> MEKVFYVTTPIYYVNAEPHLGHAYTTVVADFLARWHRLDGYRTFFLTGTDEHGETVYRAAQAAGEDPKAFVDRVSGRFKRAWDLLGIAYDDFIRTTEERHKKVVQLVLKKVYEAGDIYYGEYEGLYCVSCERFYTEKELVEGLCPIHGRPVERRKEGNYFFRMEKYRPWLQEYIQENPDLIRPEGYRNEVLAMLAEPIGDLSISRPKSRVPWGIPLPWDENHVTYVWFDALLNYVSALDYPEGEAYRTFWPHAWHLIGKDILKPHAVFWPTMLKAAGIPMYRHLNVGGFLLGPDGRKMSKTLGNVVDPFALLEKYGRDALRYYLLREIPYGQDTPVSEEALRTRYEADLADDLGNLVQRTRAMLFRFAEGRIPEPVAGEELAEGTGLAGRLR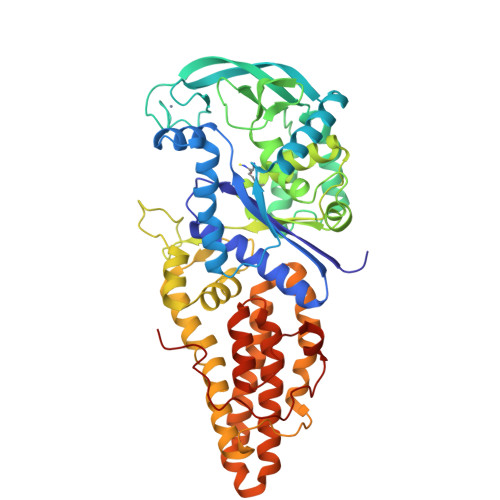PLVRELKFHVALEEAMAYVKALNRYINEKKPWELFKKEPEEARAVLYRVVEGLRIASILLTPAMPDKMAELRRALGLKEEVRLEEAERWGLAEPRPIPEEAPVLFPKKEA>[2x]MISLADLQRRIETGELSPNAAIAQSHAAIEAREKEVHAF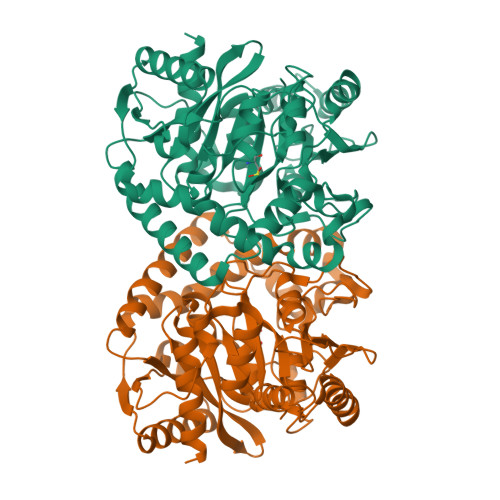VRHDKSARAQASGPLRGIAVGIKDIIDTANMPTEMGSEIYRGWQPRSDAPVVMMLKRAGATIIGKTTTTAFASRDPTATLNPHNTGHSPGGSSSGSAAAVGAGMIPLALGTQTGGCVIRPAAYCGTAAIKPSFRMLPTVGVKCYSWALDTVGLFGARAEDLARGLLAMTGRSEFSGIVPAKAPRIGVVRQEFAGAVEPAAEQGLQAAIKAAERAGASVQAIDLPEAVHEAWRIHPIIQDFEAHRALAWEFSEHHDEIAPMLRASLDATVGLTPKEYDEARRIGRRGRRELGEVFEGVDVLLTYSAPGTAPAKALASTGDPRYNRLWTLMGNPCVNVPVLKVGGLPIGVQVIARFGNDAHALATAWFLEDALAKSG> MLNGPSIIISLFFCFVSGAYACCKCDCQSGWEWFGGSCYLFDETERGWEDSKTFCESQNAALVTVESSEEDDFIRGVISAQSAFHYYWIGGSWDAEHSEYRWIDGSSISFNGWGPNRPDADEGCMDYLNYKEIVWQWNDHQDCVNTKGPSICETDCSE;> MLNGASIIVSLFLCFVGGAYACCSEDDCPSGWKFFGGSCYLFDEGSRGWEGSKAFCESKDASLVTVE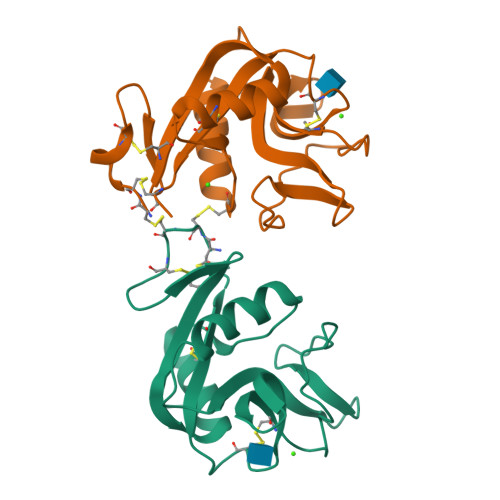CSKEDDFIRGILSGQTAKHYYWIGARWNEEHNDYRWIDGSPFTFIGWGPGKPDNNKGCLDYLNYKEVVWQWNDHVDCENTNGPCICEIDCSD>[2x]MSLSGALKENSGKPSEVEYTHFKDLQALEMERGRLYETIVVTWDDSMVGNAAPIGVLCTGDDTVTLYLYQGTRTVENVLNNGRFTVNVTLDPLIFTDSTLGDLEED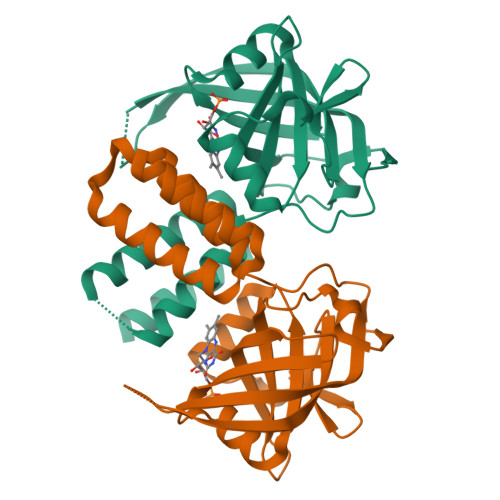MFSHYRDFLHLRGADAFFTAEVVSVKKLVKRDRFGESELHVVKARAGDVMRAESFRMALNRGIYAVIESLIAYTRAEFSDPLVLRERIAEMNRVARKVGGPREKEAMRRIIQALESKISEGHHHHHH>[2x]MGSSHHHHHHSSGLVPRGSAEFHDVTEQQKIDNDRKQFVSNVSHELRTPLTSLRSYIEALSDGAWKDPEVAPGFLKVTQEETDRMIRMINELLSLSRMDSGTTRVDMELVNINEMFNYVLDRFDMILKKDDNPAKYYTIKREFTKRDLWVEIDTDKFTQVLDNIMNNAIKYSPDGGVVTCRLLETHNQVIISISDQGLGIPRADLGHVFDRFFRVDKARSRAQGGTGLGLAISKEVVQMLGGRIWVDSVEGKGSTFYISLPYEPYEEEDLWDDDSQA

A typical TCS is composed of a sensor histidine kinase (SK) and a cognate response regulator (RR), which are encoded by genes that are often clustered in the genome. Modulated by stimulating signals, an SK first performs an autokinase activity and phosphorylates a conserved histidine in its DHp domain. Here, we sought to determine the crystal structures of a WalK homologue, lpWalK from Lactobacillus plantarum, which shares 60% sequence identity in the DHp and CA domains to our previous solved smVicK structure, in different conformations in the presence of ATP analogues or ADP. The catalytic region of lpWalK contains one DHp domain (amino acids 370–450) and one CA domain (amino acids 450–624).

However, the overall structure showed the same conformation as lpWalK co-crystallized with AMPPCP. Indeed, we also observed the same conformation for lpWalK that was crystallized in the presence of ADP. Interestingly, the interaction between Lys476 and Ala406 in lpWalK is not found in smVicK as Lys476 is substituted by Gln301. Together, our data indicate that WalK adopts a closed structure in the presence of ATP analogues or ADP, which is characterized by the asymmetric positioning of the two CA domains; only one monomer of the dimer switches to a closed conformation while the other one remains open. The adenine plane of ADP is sandwiched by Tyr518 from the N box on one side and by Ile547 from the G1 box and Phe603 from β7 on the other, and is further fixed by a hydrogen bond between Asp542 and the amine at adenine C6. The α-phosphate (αP) forms hydrogen bonds to the amine of Asn514 and the main chain of residues 574–577 from the G2 box. The β-phosphate (βP) forms hydrogen bonds to Gly572 and Thr573 from the G2 box. ATP/ADP fits into the active site of the CA domain through extensive interactions involving the N box and the G1 and G2 loops. We have found that ATP/ADP interacts with His391 in the DHp domain through hydrogen bonds in the closed lpWalK. AMP has extremely weak binding abilities. In agreement with these results, a recent report has indicated that ADP rather than AMP is an efficient VicK kinase inhibitor.> GPLGSPEFMINGVSLQGTAGYEAHTEEGNVNVKKLLESLNSKSLGDMDKDSELAATLQKMINPSGGDGNASGCALHACMAMLGYGVREAPVPNEISEYMTGFFHRHLEQIDSEGIVSHPNETYSKFRERIAENILQNTSKGSVVMISIEQATHWIAGFNDGEKIMFLDVQTGK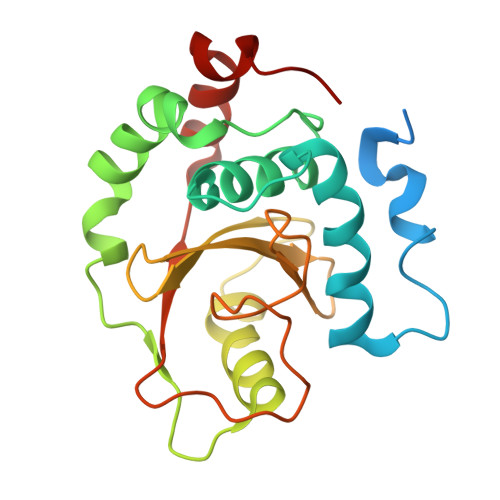GFNLYDPVEKSPDAFVDENSSVQVIHVSDQEFDHYANSSSWKSKRLC> MDDLTIEILTDDADYDLQRFDCGEEALNLFLTTHLVRQHRNKILRAYILCRNTPERQVLGYYTLCGSCFERAALPSKSKQKKIPYKNIPSVTLGR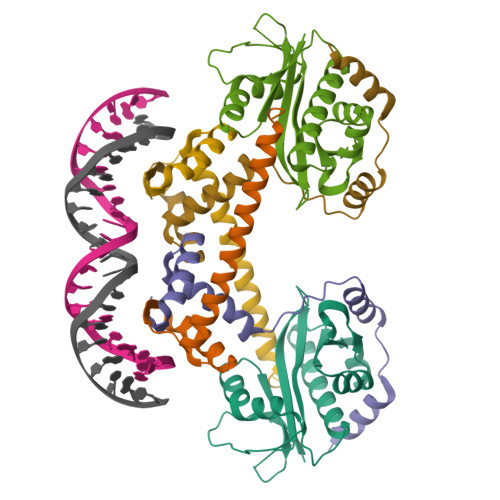LAIDRSLQGQGWGATLVAHAMKVVWSASLAVGIHGLFVEALNEKAHTFYKSLGFIPLVGENENALFFPTKSIELLFTQSD;>MSAVKKQRIDLRLTDDDKSMIEEAAAISNQSVSQFMLNSASQRAAEVIEQHRRVILNEESWTRVMDALSNPPSPGEKLKRAAKRLQGM[2x]>[4x]SNAMVIPYDYIVIGGGSAGIASANRAAMHGAKVLLAEGKEIGGTCVNLGCVPKKVMWYGAQVADILGTYAKDYGFDFKEKAFDFKQLKANRQAYIDRIHASYERGFEQNGVDRIYDYAVFKDAHTVEIAGQLYTAPHILIATGGHPVFPDIEGAQYGISSDGFFALDEVPKRTAVVGAGYIAVELAGVLHALGSKTDLFIRHDRPLRSFDKTIVDVLVDEMAVNGPRLHTHAEVA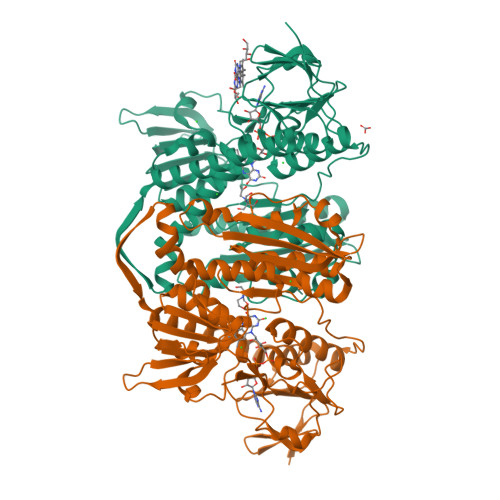KVVKNTDESLTLYLKDGQEVEVDQLIWAIGRKPNLEGFSLDKTGVTLNDKGYIETDAYENTSVKGIYAVGDVNGKLALTPVAVAAGRRLSERLFNGKTDEKLDYQNVATVIFSHPVIGSVGLSEEAAVKQYGQEAVKTYQSRFTSMFTAITNHRQPCLMKLVTVGDTEKIVGLHGIGYGVDEMIQGFAVAIKMGATKADFDNTVAIHPTGSEEFVTMR>[4x]MDIKINDITLGNNSPFVLFGGINVLESLDSTLQTCAHYVEVTRKLGIPYIFKASFDKANRSSIHSYRGVGLEEGLKIFEKVKAEFGIPVITDVHEPHQCQPVAEVCDVIQLPARLAAQTDLVVAMAKTGNVVNIKKPQFLSPSQMKNI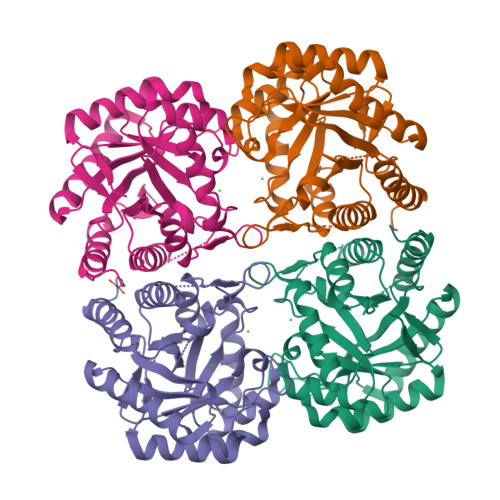VEKFHEAGNGKLILCERGSSFGYDNLVVDMLGFGVMKQTCGNLPVIFDVTHSLQTRDAGSAASGGRRAQALDLALAGMATRLAGLFLESHPDPKLAKCDGPSALPLHLLEDFLIRIKALDDLIKSQPILTIE> MVANPEHYIKHPLQNRWALWFFKNDKSKTWQANLRLISKFDTVEDFWALYNHIQLSSNLMPGCDYSLFKDGIEPMWEDEKNKRGGRWLITLNKQQRRSDLDRFWLETLLCLIGESFDDYSDDVCGAVVNVRAKGDKIAIWTTECENREAVTHIGRVYKERLGLPPKIVIGYQSHADTATKSGSTTKNRFVV;> XKKRYSRLQLLLFWX

The eukaryotic translation initiation factor 4E (eIF4E) protein is a vital component of the cap-dependent mechanism for mRNA translation. It binds the 7-methylguanosine (m7G) cap structure present at the 5′ end of mRNA molecules and recruits it as part of the eIF4F assembly which also includes two other partner proteins, eIF4A and eIF4G, to the translational machinery for protein synthesis. We have used a structure-guided approach to rationally develop a set of hydrocarbon stapled-peptides with high binding affinities and residence times against the oncogenic eukaryotic translation initiation factor 4E (eIF4E) protein. Crystal structures of these peptides in complex with eIF4E show that they form specific interactions with a region on the protein-binding interface of eIF4E which is distinct from the other well-established canonical interactions.

The lifetime of binding measured in terms of the residence time (RT = 1/koff) was also found to be higher for the 13mer peptides (∼36 seconds) compared to their 12mer counterparts (10 seconds for sTIP-05 and 6 seconds for sTIP-06). Crystal structures of the complexes of sTIP-07 and sTIP-08 with eIF4E were determined (C and Table S1†). The essential interactions made by the parent 12mer peptides were retained. More significantly, the added tryptophan (W13) in the sTIP-07 structure was observed to indeed efficiently interact with and engage the patch on eIF4E. W13 formed pi-stacking interactions with W73 and Y76 and hydrophobic interactions with L131. In addition, the amide nitrogen of the side-chain of W13 was also observed to form hydrogen-bond interaction with the side-chain of N77. The hydrophobic/aromatic interactions between W13 and the residues from the protein as observed in the sTIP-07 crystal structure were fairly stable except for the W13–N77 hydrogen-bond (occupancy < 20%, Movie S3†), which nevertheless contributed to favorable binding energy (–3.2 kcal mol–1) from this residue. Hence, the additional specific interactions formed by the residues at the extended C-terminus (W13 and &13) for sTIP-07/sTIP-08 respectively could create a greater barrier and hence result in the lower association rates observed for these peptides as compared to sTIP-05/sTIP-06.>[5x]GQDMVSPPPPIADEPLTVNTGIYLIECYSLDDKAETFKVNAFLSLSWKDRRLAFDPVRSGVRVKTYEPEAIWIPEIRFVNVENARDADVVDISVSPDGTVQYLERFSARVLSPLDFRRYPFDSQTLHIYLIVRSVDTRNIVLAVDLEKVGKNDDVFLTGWDIESFTAVVKPANFALEDRLESKLDYQLRISRQYFSYIPNIILPMLFILFISWTAFWSTSYEANVTLVVSTLIAHIAFNILVETNLPKTPYMTYTGAIIFMIYLFYFVAVIEVTVQHYLKVESQPARAASITRASRIAFPVVFLLANIILAFLFFGF

To improve the understanding of molecular interactions between xenon and transmembrane receptor targets, we investigated xenon binding with the Gloebacter violaceus ligand-gated ion channel (GLIC), a member of the pLGIC family, using X-ray crystallography under pressurized gas. Previously, the sensitivity of GLIC to gaseous anesthetics has been studied using 2-electrode voltage clamping techniques and this revealed that GLIC currents are inhibited by clinical concentrations of xenon. GLIC, whose X-ray structures has been solved in open, locally-closed (LC)–inactive- and resting-state conformations, is extensively used to identify binding sites of general anesthetics, channel blockers, alcohols, and other allosteric modulators in pLGICs. Here, we show by X-ray diffraction that xenon has multiple and specific binding sites in GLIC either in the open and LC (inactive) conformations, and that these binding sites differ between the two conformations.

Xenon-bound GLIC open and LC structures were obtained from crystals pressurized with 2 MPa (20 bar) of xenon and analysed by X-ray crystallography at 3.1 and 3.4 Å resolution respectively. In GLIC open form, xenon is found at three close but different locations in an intra-subunit cavity located in the upper half of the TMD. This cavity is lined by residues from a single subunit with contributions from helices M1 (Y197, I201, I202 and M205), M2 (V242), M3 (Y254, T255, I258 and I259), M4, the apex of the β6- β7 loop (Y119, P120, F121) and the M2-3 loop (N245). The cavity is accessible from the lipid bilayer, it penetrates the interior of the subunit along a direction that points towards the ECD-TMD interface. The first two locations of xenon are observed at the pocket entrance and were modelled as alternative poses of the same xenon atom with 0.5 occupancy each. The third xenon atom with 0.9 occupancy is deeply buried within the cavity in a highly hydrophobic environment. The xenon atoms are all engaged in van der Waals interactions with the hydrophobic side chains of surrounding residues and the alkyl chains of the lipid molecule. In GLIC open form, the intra-subunit binding site can be considered as a common anesthetic binding site, since it can bind not only xenon, but other anesthetics like propofol, desflurane or bromoform. In GLIC open form, xenon binds between M1 and M2 helices from one subunit and M2 helix from the adjacent subunit in the inner part of the TMD while in GLIC LC form, xenon binds between M1 helix from one subunit and M2 and M3 helices from the adjacent subunit in the outer part of the TMD. The second one, named minor interfacial site, is present only in the GLIC open form and is located in a small hydrophobic cavity in the middle of the TMD.>[2x]MSLSYRIDVLLFNKFETLDVFGPVEIFGNLQDDFELNFISSDGGLVESSQKVRVETSLYTRDENIEKILFVPGGSGTREKVNDDN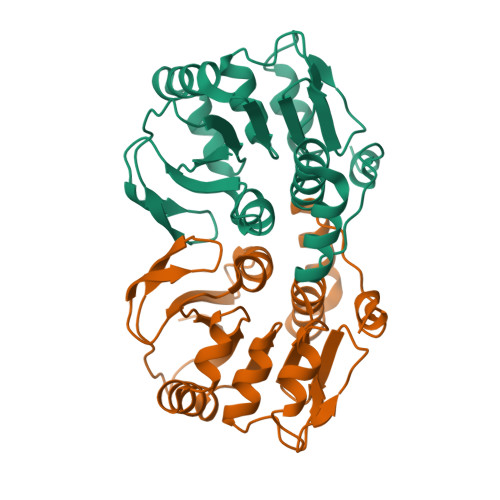FINFIGNMVKESKYIISVCTGSALLSKAGILNGKRATTNKRSFKWVTEQNEDVLWVKEARWVKDGNIYTSSGVSAGIDMTLGFIEDLIGKEKALEISRSIEYFWNEDSNYDPFSKIYGEGHHHHHH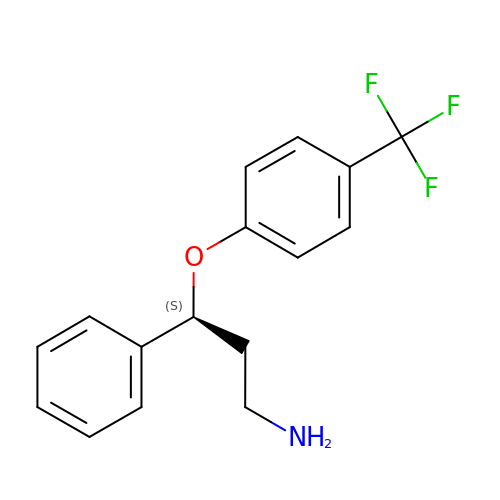(3S)-3-phenyl-3-[4-(trifluoromethyl)phenoxy]propan-1-amine | C16 H16 F3 N O | WIQRCHMSJFFONW-HNNXBMFYSA-N> MEVQPSEEEARGYIVTDRDPLRPEEGRRLVEDVARLLQVPSSAFADVEVLGPAVTFKVSANVQNVTTEDVEKATVDNK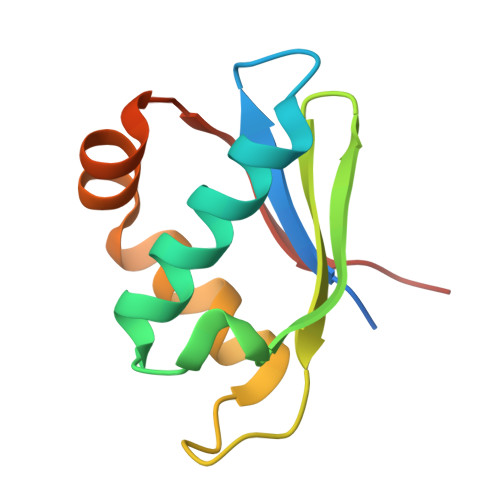DKLEETSGLKILQTGVGSKSK ethyl (2R)-2-oxidanylpropanoate | C5 H10 O3 | 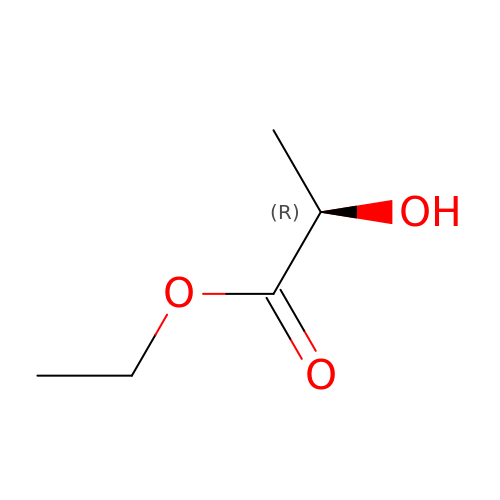LZCLXQDLBQLTDK-SCSAIBSYSA-N> MAKQYDDNECPFCDEVSKYEKLAKIGQGTFGEVFKARHRKTGQRVALKKVLMENEKEGFPITALREIKILQLLKHENVVNLIEICRTKASPYNRCKGSIYLVFDFCEHDLAGLLSNVLVKFTLSEIKRVMQMLLNGLFYIHRNKILHRDMKAANVLITRDGVLKLADFGLARA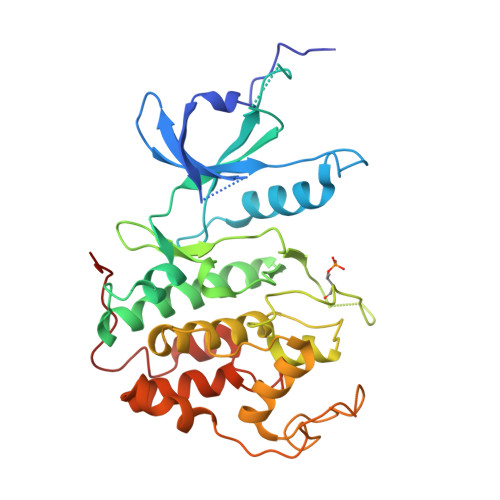FSLAKNSQPNRYTNRVVTLWYRPPELLLGERDYGPPIDLWGAGCIMAEMWTRSPIMQGNTEQHQLALISQLCGSITPEVWPNVDNYELYEKLELVKGQKRKVKDRLAAYVRDPYALDLIDKLLVLDPAQRIDSEDALEHDFFWSDPMPSDLKGMLST>[2x]GSHMGSGQVTLDFFQFKAEAADWFKQAAQEFEKENPDIRININNSANAQTDLRTRFVKDRVPDVITFNGDYSFGTFAASGVFHDFTDDPLVSEL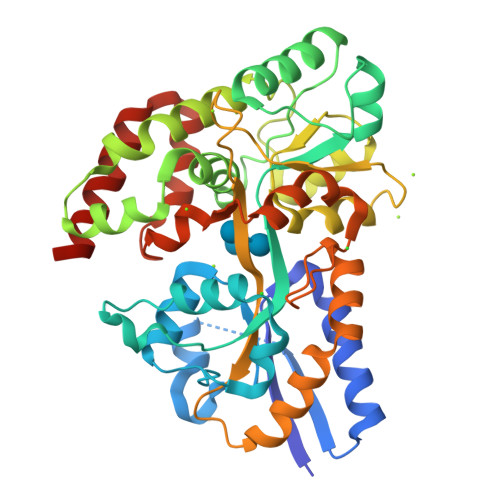NEGMVNIAKNLVQTSDPAKKRLYGLPFAGNASGYIYNKDLFRKVGLDPDNPPQTWDEFIAMLKKFRDAGINPVQATLADAWTTQAPLASLAGTLVPESEYAALKSGDTTFKQIWTEPIEKEIELFKYADSEKGVTYQQGTQNFAKGTAAIIPLGTYAIPQITMVNKDIDLGFAQMPATNDASKQILTAGDDVILTMGANSRHKEQSMRFIRFLMSKKQLENYADAQSAITPLKETYFGNKALEPVRPFFESNRVADFCDHYIPSSINIGGYLQSAIMSGNVNQFIDSMQNEWNKVQARDFRK> MGSSHHHHHHSSGRENLYFQGMIKEMIEDFISKGGLIFTHSGRYTNT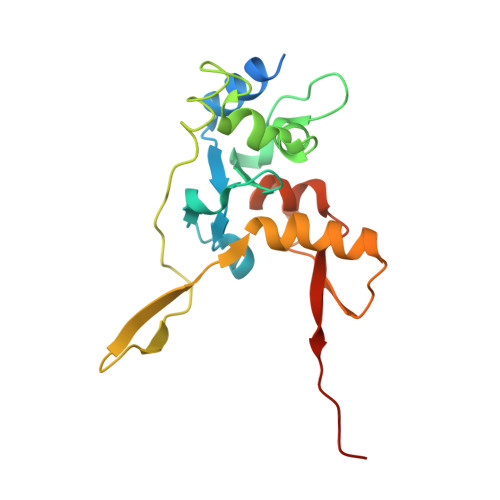NNSCFIFNKNDIGVDTKVDMYTPKSAGIKNEEGENLWQVLNKANMFYRIYSGELGEELQYLLKSCCTAKEDVTTLPQIYFKNGEGYDILVPIGNAHNLISGTEYLWEHKYYNTFTQKLGGSNPQNCTHACNKMRGGFKQFNCTPPQVEDNYNA>[2x]SRNVPFPYAETDVADLQARMTAGELDSTTLTQAY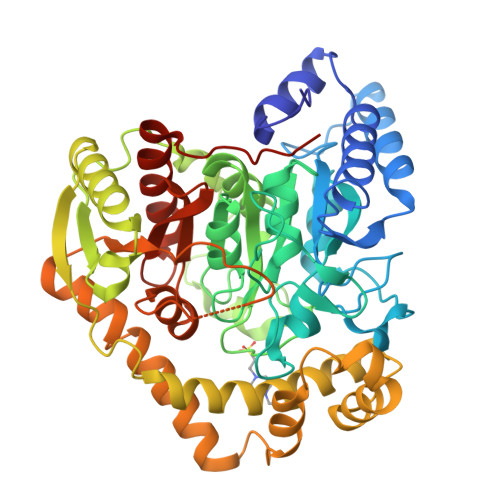LQRIAALDRTGPRLRAVIELNPDALKEAAERDRERRDGRLRGPLHGIPLLLKDNINAAPMATSAGSLALQGFRPDDAYLVRRLRDAGAVVLGKTNLSEWANFRGNDSISGWSARGGQTRNPYRISHSPCGSSSGSAVAVAANLASVAIGTETDGSIVCPAAINGVVGLKPTVGLVSRDGIIPISFSQDTAGPMARSVADAAAVLTAIAGRDDADPATATMPGRAVYDYTARLDPQGLRGKRIGLLQTPLLKYRGMPPLIEQAATELRRAGAVVVPVELPNQGAWAEAERTLLLYEFKAGLERYFNTHRAPLRSLADLIAFNQAHSKQELGLFGQELLVEADATAGLADPAYIRARSDARRLAGPEGIDAALAAHQLDALVAPTTGVAWPIRSEGDDFPGESYSAAAVAGYPSLTVPMGQIDGLPVGLLFMGTAWSEPKLIEMAYAYEQRTRARRPPHFDTDALIDAGEP>[3x]KDRPDFCELPAD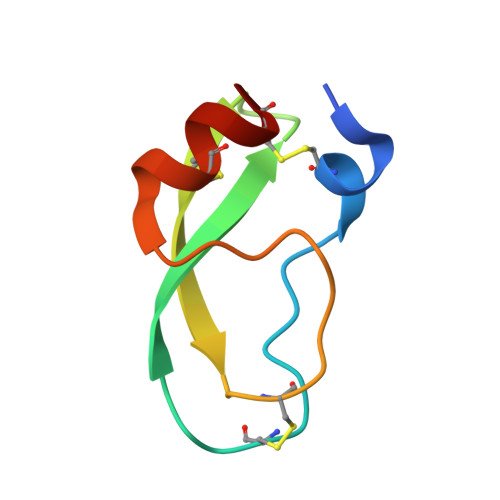TGPCRVRFPSFYYNPDEKKCLEFIYGGCEGNANNFITKEECESTCAA>[2x]AALTEKTDIFESGRNGKPNKDGIKSYRIPALLKTDKG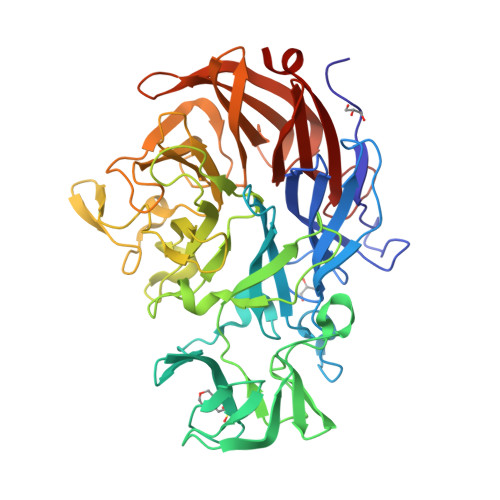TLIAGADERRLHSSDWGDIGMVIRRSEDNGKTWGDRVTITNLRDNPKASDPSIGSPVNIDMVLVQDPETKRIFSIYDMFPEGKGIFGMSSQKEEAYKKIDGKTYQILYREGEKGAYTIRENGTVYTPDGKATDYRVVVDPVKPAYSDKGDLYKGNQLLGNIYFTTNKTSPFRIAKDSYLWMSYSDDDGKTWSAPQDITPMVKADWMKFLGVGPGTGIVLRNGPHKGRILIPVYTTNNVSHLNGSQSSRIIYSDDHGKTWHAGEAVNDNRQVDGQKIHSSTMNNRRAQNTESTVVQLNNGDVKLFMRGLTGDLQVATSKDGGVTWEKDIKRYPQVKDVYVQMSAIHTMHEGKEYIILSNAGGPKRENGMVHLARVEENGELTWLKHNPIQKGEFAYNSLQELGNGEYGILYEHTEKGQNAYTLSFRKFNWDFLSK> MRVLLAPMEGVLDSLVRELLTEVNDYDLCITEFVRVVDQLLPVKVFHRICPELQNASRTPSGTLVRVQLLGQFPQWLAENAARAVELGSWGVDLNCGCPSKTVNGSGGGATLLKDPELIYQGAKAMREAVPAHLPVSVKVRLGWDSGEKKFEIADAVQQAGATELVVHGRTKEQGYRAEHIDWQAIGDIRQRL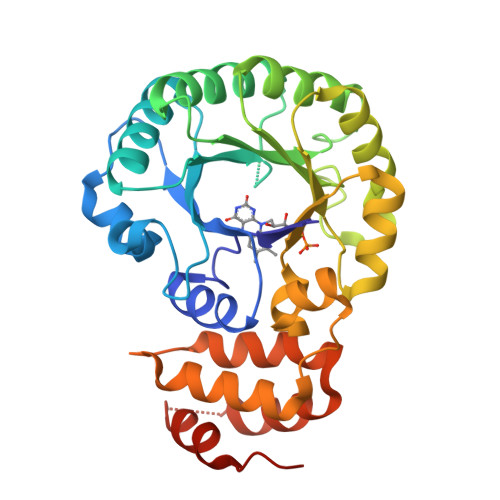NIPVIANGEIWDWQSAQQCMAISGCDAVMIGRGALNIPNLSRVVKYNEPRMPWPEVVALLQKYTRLEKQGDTGLYHVARIKQWLSYLRKEYDEATELFQHVRVLNNSPDIARAIQAIDIEKLEHHHHHH> MLKQVEIFTDGSCLGNPGPGGYGAILRYRGREKTFSAGYTRTTNNRMELMAAIVALEALKEHCEVILSTDSQYVRQGITQWIHNWKKRGWKTADKKPVKNVDLWQRLDAALGQHQIKWEWVKGHAGHPENERCDELARAAAMNPTLEDTGYQVEV

The ribonuclease (RNase) H family of enzymes catalyze the specific cleavage of RNA strands of RNA/DNA hybrid duplexes and play an important role in DNA replication and repair. RNase H cleaves the phosphodiester bonds of RNA in double-stranded DNA/RNA hybrids, leaving 3′-hydroxyl and 5′-phosphate groups at each cleaved site. This catalysis requires divalent cations such as Mg2+, Mn2+ and Zn2+. Structural analyses found that the DEDD motif coordinates the divalent cation at the active site, acting as metal ligands, and constitutes the pivotal scaffold for the catalytic reaction. In addition to the highly conserved DEDD motif, a histidine adjacent to the active site (His124 in E. coli RNase HI) in the loop structure between β5 and α5 has also frequently been discussed.

In the RNH_Mg_2 structure an Mg2+ ion is bound in a different position to those in the other two structures, RNH_Mg_1 and RNH_Mg_3, which are very similar to each other. The exact reason for the observed variation in the binding of the Mg2+ ion is unknown.>[2x]PGSKPFSVPVLTVEEMTNSRFPIPLEKLFTGPSSAFVVQPQNGRCTTDGVLLGTTQLSPVNICTFRGDVTHITGSRNYTMNLASQNWNDYDPTEEIPAPLGTPDFVGKIQGVLTQTTRTDGSTRGHKATVYTGSADFAPKLGRVQFETDTDRDFEANQNTKFTPVGVIQDGGTTHRNEPQQWVLPSYSGRNTHNVHLAPAVAPTFPGEQLLFFRSTMPGCSGYPNMDLDCLLPQEWVQY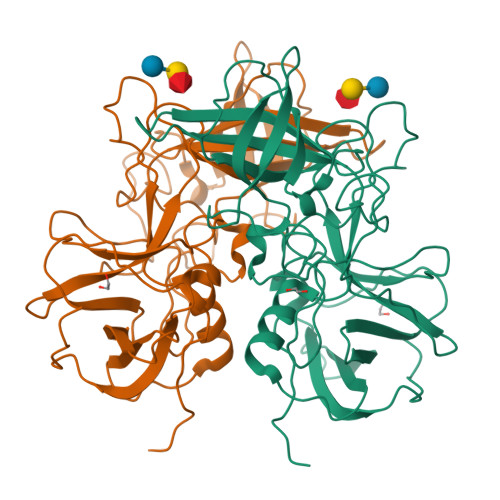FYQEAAPAQSDVALLRFVNPDTGRVLFECKLHKSGYVTVAHTGQHDLVIPPNGYFRFDSWVNQFYTLAPM> MQGHPEVI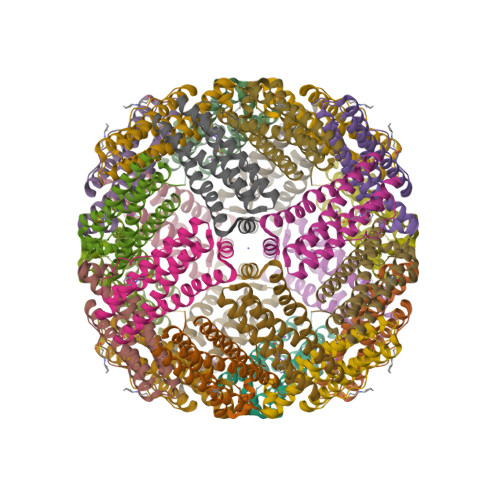DYLNTLLTGELAARDQYFIHSRMYEDWGFSKLYERLNHEMEEETQHADALLRRILLLEGTPRMRPDDIHPGTTVPEMLEADLKLERHVRAALAKGIALCEQHKDFVSRDILKAQLADTEEDHAYWLEQQLGLIARMGLENYLQSQI>MASDYEAVNTNPYGVSDGELGPLKYGARFMNMQQRVIPIGSPSLTTGPGNDLQNTDLISSGNYIGYFGNNNNWGFNNEANWNFTDSRMNYAYQNFYSQIFLPWNEIYEIAKDSDSPSEQAILEIANIVRNIAWLRATDVFGPIAYNSAGDGSIAPKFDSQEVVYRSMLADLSKSVELLNTISYSVMAQYDLIYNGNVQNWVKLANSLMLRIVVRVHFIDETLAKEYITKALDPKNGGVIEDISSEAKIKSSDKMPLLNSMLASVNEYNETRMGATIWGYLDGYKDPRLSAYFTEGTYGSGSWAQTGYFPVAPTNSKSKSETSYSAKFASRPKVDSNSPLYWFRASETYFLKAEAALYNLIGGDP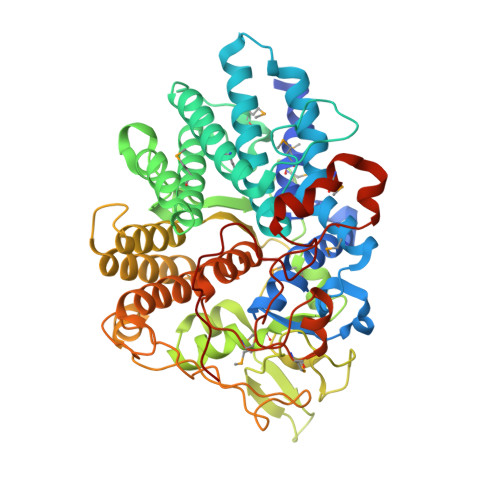KTFYEQGINISFQEQGVSGVATYLSGTGKPTGLTGSNYKYGTYNHDLSIGNTSPKWDDYTGNLSKQEEQLQKIITQKYLALYPNAVEAWTEYRRTGFPYLMKPMDEAAPGRIGASIEDCRVPERFRFAPTAYNSNPNMAEIPTLLGGGDIGATKLWWVRSNRPKQPNQ[2x]> MVQISEVRGNTRDHRTAAHTHIK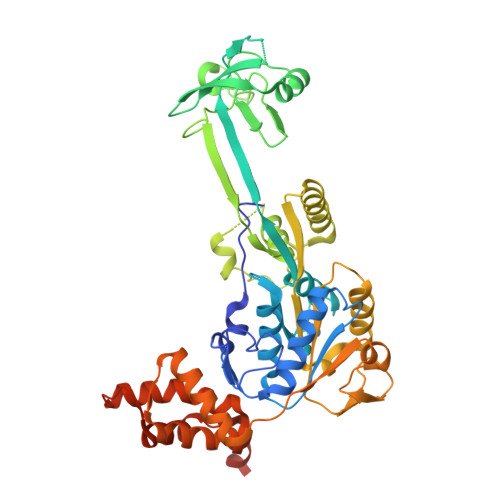GLGLNSSGIAEKQAAGFVGQCAAREACGVVVDLIKAHKMAGRGVLLAGGPGTGKTALALAISQELGTKIPFCPITGSEIYSTEVKKTEVLMENFRRAIGLRVRETKDVYEGEVTEMTPEEAENPLGGYGKTISTLLIGLKSARGQKKLRLDPSIYEAIQKERVQVGDVIYIETNTGACKRVGRSDAYATEFDLEAEEYVPIPKGEVHKKKEIVQDVTLHDLDVANARPQGGQDIISMMGQLMKPKMTEITDKLRMEINKVVQKYINQGVAELIPGVLFIDEAHMLDIECFTYLNKALESPIAPIVVLASNRGIATIRGADDLKAAHGIPPDFLQRLLIIPTHPYEPDEIRRIVRIRAQTEGVQLTDAAVDRVAEHGVRISLRYCLQLLAPASILARVNGRTQVDVQDIAEAEELFLDARRSANILTSTGESGGLHGFIS Zorbamycin | C55 H85 N19 O21 S2 | 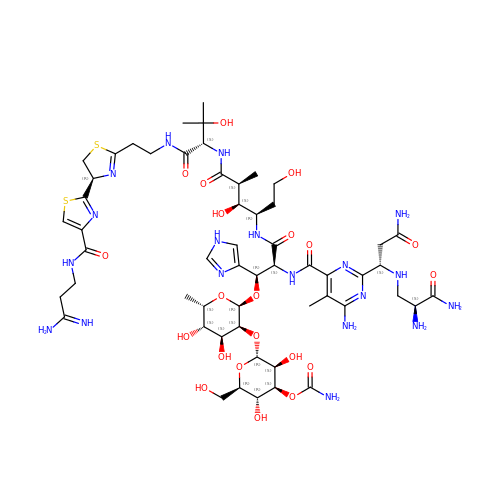UJKRUPHWCPAJIL-CPLCKGKLSA-N> PFPWNKIRLPEYVIPVHYDLLIHANLTTLTFWGTTKVEITASQPTSTIILHSHHLQISRATLRKGAGERLSEEPLQVLEHPRQEQIALLAPEPLLVGLPYTVVIHYAGNLSETFHGFYKSTYRTKEGELRILASTQFEPTAARMAF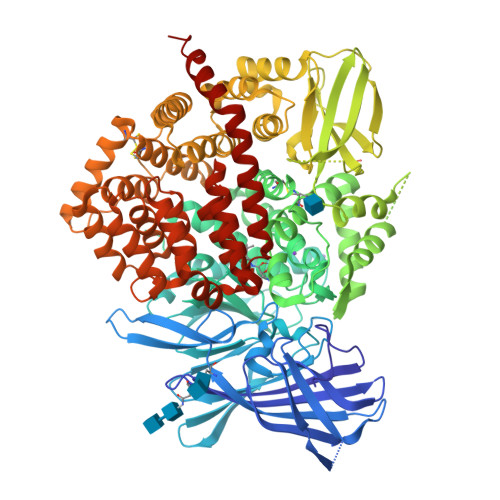PCFDEPAFKASFSIKIRREPRHLAISNMPLVKSVTVAEGLIEDHFDVTVKMSTYLVAFIISDFESVSKITKSGVKVSVYAVPDKINQADYALDAAVTLLEFYEDYFSIPYPLPKQDLAAIPDFQSGAMENWGLTTYRESALLFDAEKSSASSKLGITMTVAHELAHQWFGNLVTMEWWNDLWLNEGFAKFMEFVSVSVTHPELKVGDYFFGKCFDAMEVDALNSSHPVSTPVENPAQIREMFDDVSYDKGACILNMLREYLSADAFKSGIVQYLQKHSYKNTKNEDLWDSMASICPTDGVKGMDGFCSRSQHSSSSSHWHQEGVDVKTMMNTWTLQKGFPLITITVRGRNVHMKQEHYMKGSDGAPDTGYLWHVPLTFITSKSDMVHRFLLKTKTDVLILPEEVEWIKFNVGMNGYYIVHYEDDGWDSLTGLLKGTHTAVSSNDRASLINNAFQLVSIGKLSIEKALDLSLYLKHETEIMPVFQGLNELIPMYKLMEKRDMNEVETQFKAFLIRLLRDLIDKQTWTDEGSVSERMLRSQLLLLACVHNYQPCVQRAEGYFRKWKESNGNLSLPVDVTLAVFAVGAQSTEGWDFLYSKYQFSLSSTEKSQIEFALCRTQNKEKLQWLLDESFKGDKIKTQEFPQILTLIGRNPVGYPLAWQFLRKNWNKLVQKFELGSSSIAHMVMGTTNQFSTRTRLEEVKGFFSSLKENGSQLRCVQQTIETIEENIGWMDKNFDKIRVWLQSEKLERKK Rab proteins, the biggest subfamily within the superfamily of small GTPases, are major regulators of vesicular trafficking in eukaryotic cells. One such family of effector proteins that was reported to link Rab proteins and the cytoskeleton is the Mical (molecules interacting with CasL) family. In this publication, we present a thorough biochemical and structural analysis of a Rab effector domain termed bivalent Mical/EHBP Rab binding (bMERB) domain. The results show that the domains probably constitute a Rab8-effector family involved in endosomal trafficking, and the Rab-binding specificity can be well explained from the 3-dimensional structures of complexes determined in this work.

Interestingly, whereas Rab1 contains a glutamate near the N-terminus (Glu4), all Rab8 family members contain one or (in the case of Rab10) two lysine residues in this region that point towards a negatively charged patch in Mical-cL. We therefore tested whether these N-terminal residues of the Rab proteins might determine the specificity of bMERB domains towards Rab8 and its homologues rather than Rab1. We constructed a chimera of Rab1 containing the 4 N-terminal aa of Rab8, thus exchanging the negatively charged glutamate for a positively charged lysine. The x-ray crystallographic structure of this Rab1 chimera (termed Rab1R8N) in complex with Mical-cL clearly showed that the helices 1 and 2 move closer and adopt a similar conformation as observed in the structures of Rab8:Mical-cL and Rab10:Mical-cL. Additionally, ITC measurements showed that the chimera had an approximately five-fold increased binding affinity compared to Rab1. In contrast to Rab1, the chimera Rab1R8N bound both EHBP1 and EHBP1L1 in aSEC experiments, thus clearly indicating that the N-terminus is important for the interaction and contributes to the observed specificity of bMERB domains towards Rab proteins. However, after mutating the 4 N-terminal residues of Rab1 to the corresponding sequence of Rab8 (the resulting chimera is called Rab1R8N), the structure of Rab1R8N:Mical-cL shows a similar conformation of α-helices 1 and 2 as in the structure of Rab8:Mical-cL. (c) Consistently, ITC measurements show that the affinity of binding increases approximately five-fold after mutating the N-terminal residues (Rab1:Mical-cL: KD = 5.2 µM; Rab1R8N:Mical-cL: KD = 1.1 µM; Rab8:Mical-cL: KD = 0.23 µM). In this regard, we showed that the N-terminal residues preceding the RabSF1 motif contribute to this specificity, an observation that has previously not been made in other Rab:effector interactions.

> GHMKQEELKRLYKAQAIQRQLEEVEERQRASEIQGVRLEKALRGEADSGTQDEAQLLQEWFKLVLEKNKLMRYESELLIMAQELELEDHQSRLEQKLREKMLKEESQKDEKDLNEEQEVFTELMQVIEQRDKLVDSLEEQRIREKAEDQHFES;> GHMAKTYDYLFKLLLIGDSGVGKSCLLLRFADDTYTESYISTIGVDFKIRTIELDGKTIKLQIWDTAGQERFRTITSSYYRGAHGIIVVYDVTDQESYANVKQWLQEIDRYASENVNKLLVGNKSDLTTKKVVDNTTAKEFADSLGIPFLETSAKNATNVEQAFMTMAAEIKKRMGPGAASGGERPNLKIDSTPVKPAGGGCC> GSHHPFTAQIVAVTASGYDSEKGHVPANIADGDVKTRWAASGESWVQLELDKEQSIENILIVPFKPTERKLKFSIFYSNDGKNWQPLAEGLETSSADK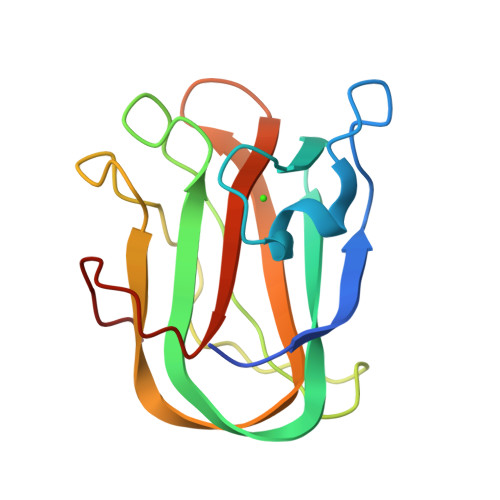NGEKLTFTPVTAKYIKLDTFGTDVNNWSAINEIAINSAAALPSRAIK> KRNKPGKATGKGKPVNNKWLNNAGKDLGSPVPDRIANKLRDKEFKSFDDFRKKFWEEVSKDPELSKQFSRNNNDRMKVGKAPKTRTQDVSGKRTSFELHHEKPISQN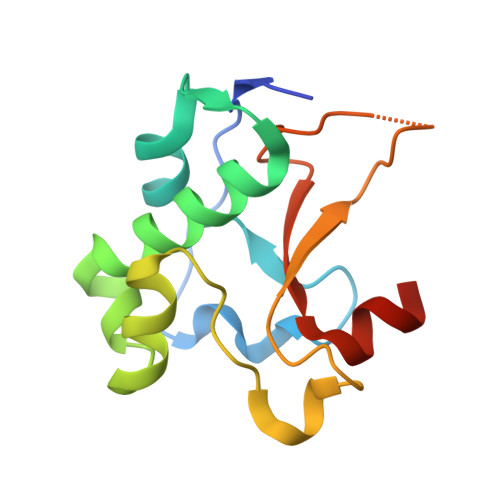GGVYDMDNISVVTPKRHIDIARGK> GGAGAGA;> UCUC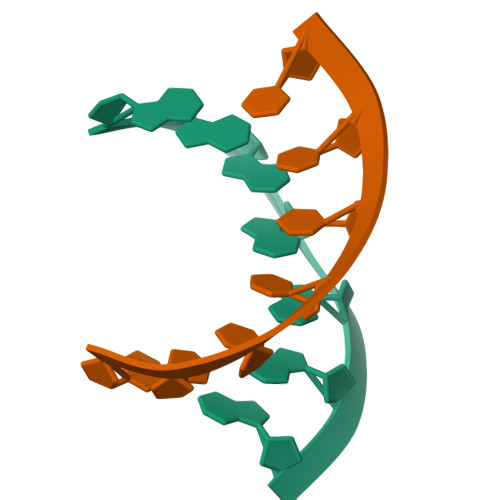UCC>[5x]MAEESFYGVTLTAESDSVTWDVDEDYARGQKLVIKQILLGAEAKENEFNVVEVNTPK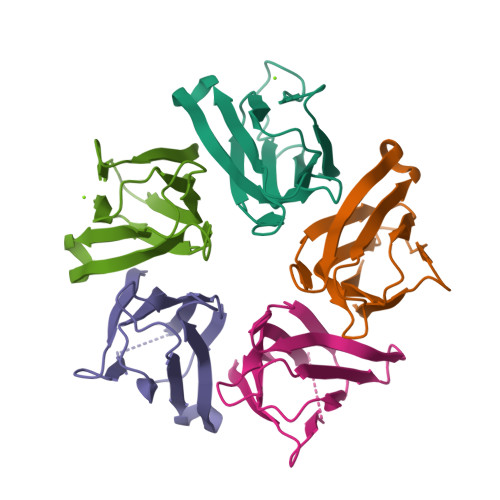DSVQIPIAVLKAGETRAVNPDVEFYESKVTFKLIKGSGPVYIHGHNIKDDV>[20x]MVVI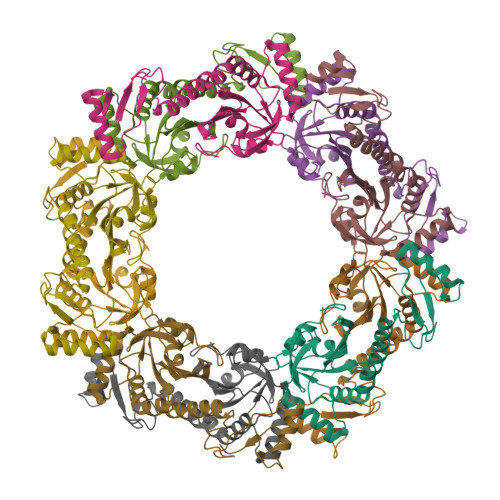GEKFPEVEVKTTHGVIKLPDYFTKQGKWFILFSHPADFTPVSTTEFYGMQKRVEEFRKLGVEPIGLSVDQVFSHIKWIEWIKDNLSVEIDFPVIADDRGELAEKLGMIPSGATITARAVFVVDDKGIIRAIVYYPAEVGRDWDEILRLVKALKISTEKGVALPHKWPNNELIGDKVIVPPASTIEEKKQREEAKAKGEIESYDWWFSYKKLE(1R,4S,5S,6S)-4-aminospiro[bicyclo[3.1.0]hexane-2,1'-cyclopropane]-4,6-dicarboxylic 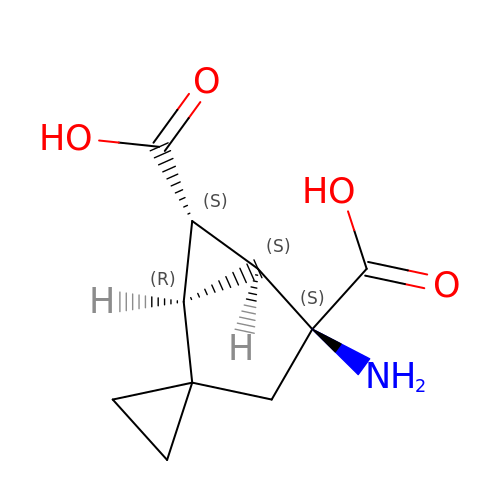acid | C10 H13 N O4 | ADTIUNVCKYGIIN-AZOMRORLSA-N> MSALSLLILGLLMAVPPASCQQGLGNLQPWMQGLIAVAVFLVLVAIAFAVNHFWCQEEPEPAHMILTVGNKADGVLVGTDGRYSSMAASFRSSEHENAYENV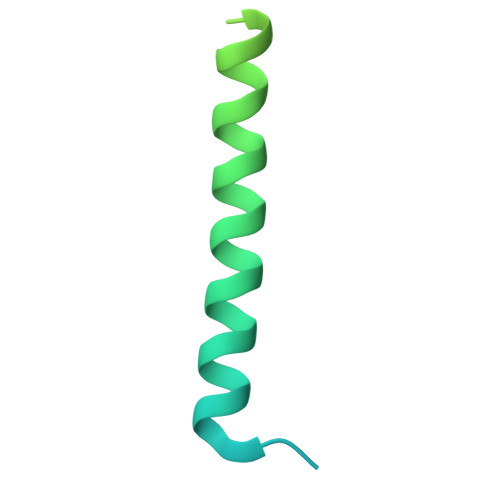PEEEGKVRSTPM>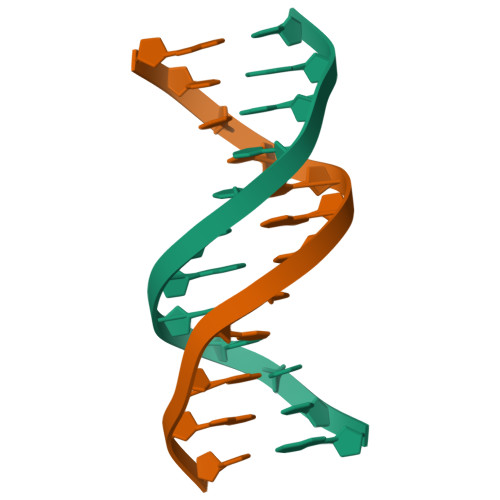ACCGAATTCGGT[6x]>APAANPAVTESVAPTTAPAPAAAAPESITPVNPAPTIQPPETRGMDLSIWGMYQHADAVVKAVMIGLVLASIVTWTILFAKGSELLRAKRRLRREQLALAEARSLDEASELAQNFSPESVSAVLLNDAQNELELSAESNDNN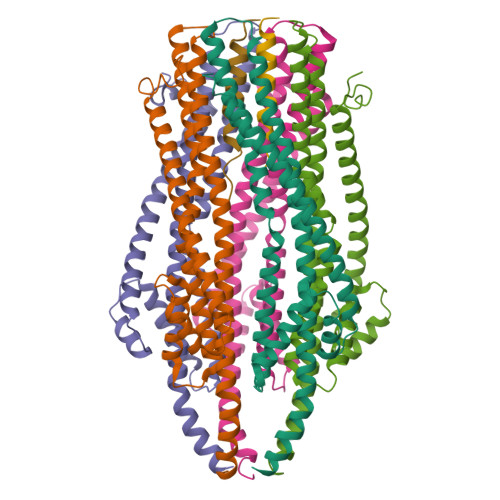GIKERTGFRLERRVAAYSRNMGRGNGFLATIGAISPFVGLFGTVWGIMNSFIGIAHSQTTNLAVVAPGIAEALLATAMGLVAAIPAVVIYNIFARVISGHRAQVGDVAAQVLLLQGRDLDLAATAEAKRSQHAHQLRAG[5x];>[2x]MAMRLNEDLDDSGELHEINVTPFIDVMLVLLIIFMVAAPLATVDIRVDLPASSAKPQPRPEKPVFLSVKADKQLYVGDQPVNADQLTSVLDQRTQANKETTIFFQADKSVDYETLMSVMDTLRKAGYLKVGLVGMEGAAKHHHHHH(2S,3S)-3-AMINO-4-[(3S)-3-FLUOROPYRROLIDIN-1-YL]-N,N-DIMETHYL-4-OXO-2-(TRANS-4-[1,2,4]TRIAZOLO[1,5-A]PYRIDIN-5-YLCYCLOHEXYL)BUTANAMIDE | C22 H31 F N6 O2 | 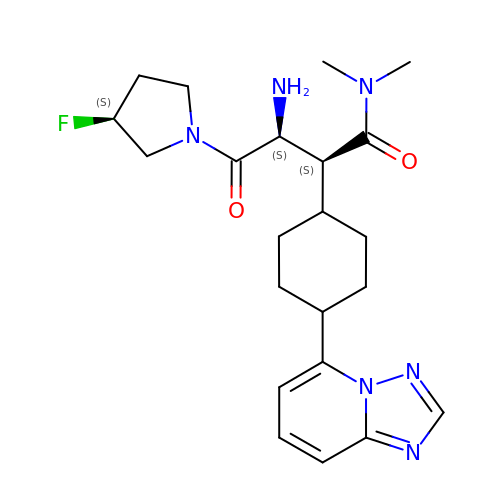ZPWDKZWKUOYOHA-UKSSEWCLSA-N>[2x]SNAMKRSIEDTPIVLIGAGNLATNLA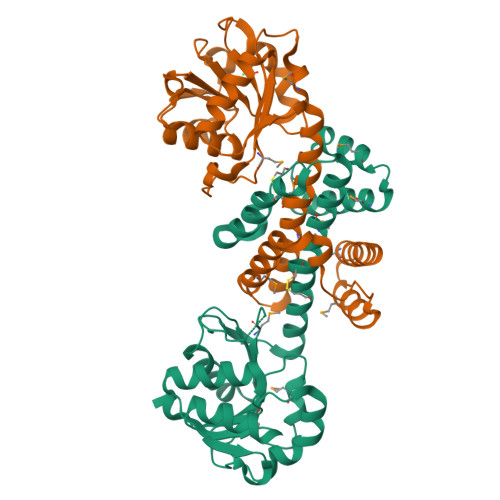KALYRKGFRIVQVYSRTEESARELAQKVEAEYTTDLAEVNPYAKLYIVSLKDSAFAELLQGIVEGKREEALMVHTAGSIPMNVWEGHVPHYGVFYPMQTFSKQREVDFKEIPFFIEASSTEDAAFLKAIASTLSNRVYDADSEQRKSLHLAAVFTCNFTNHMYALAAELLKKYNLPFDVMLPLIDETARKVHELEPKTAQTGPAIRYDENVIGNHLRMLADDPAMQRLYELLSRSIHERQ> MLNQELELSLNMAFARAREHRHEFMTVEHLLLALLSNPSAREALEACSVDLVALRQELEAFIEQTTPVLPASEEERDTQPTLSFQRVLQRAVFHVQSSGRNEVTGANVLVAIFSEQESQAAYLLRKHEVSRLDVVNFISHGT;> MGKTNDWLDFDQLAEEKVRD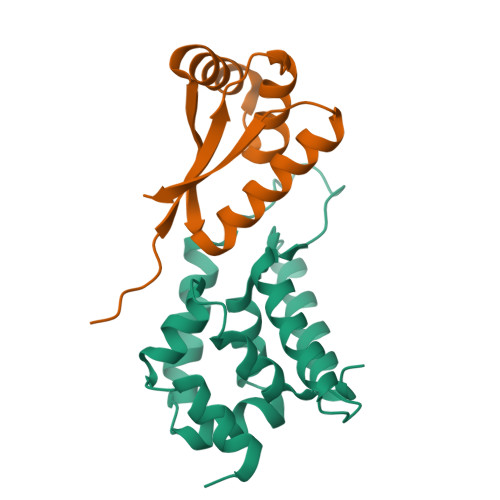ALKPPSMYKVILVNDDYTPMEFVIDVLQKFFSYDVERATQLMLAVHYQGKAICGVFTAEVAETKVAMVNKYARENEHPLLCTLEKA1-[(1S,5S,6S)-6-methyl-6-{[(6M,8R)-6-(1-methyl-1H-pyrazol-4-yl)pyrazolo[1,5-a]pyrazin-4-yl]oxy}-2-azabicyclo[3.2.0]heptan-2-yl]propan-1-one | 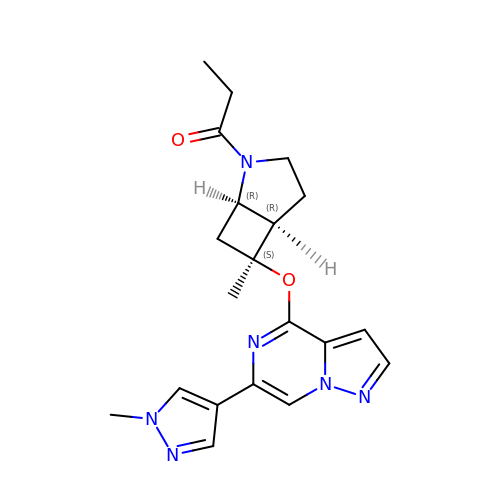C20 H24 N6 O2 | AJJZIJYLCBVMRU-DRWNPLCXSA-N N,N'-BIS(2,3-BUTADIENYL)-1,4-BUTANE-DIAMINE | C12 H20 N2 | 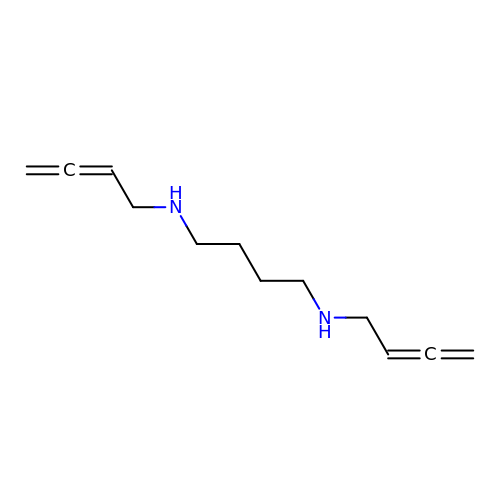IKSQCMLJDHRWOA-UHFFFAOYSA-N>GPESQLDLRVQELIKLICNVQAMEEMMMEMKYNTKKAPLGKLTVAQIKAGYQSLKKIEDCIRAGQHGRALMEACNEFYTRIPHDFGLRTPPLIRTQKELSEKIQLLEALGDIEIAIKLVKSERQGLEHPLDQHYRNLHCALRPLDHESYEFKVISQYLQSTHAPTHSDYTMTLLDLFEVEKDGEKEAFREDLHNRMLLWHGSRMSNWVGILSHGLRIAPPEAPITGYMFGKGIYFADMSSKSANYCFASRLKNTGLLLLSEVALGQCNELLEANPKAEGLLQGKHSTKGLGKMAPSSAHFVTLNGSTVPLGPASDTGI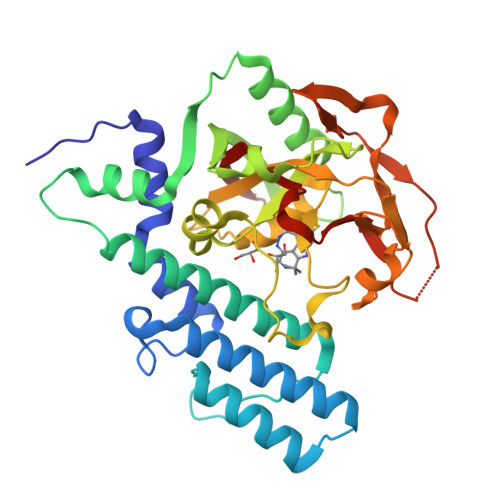LNPDGYTLNYNEYIVYNPNQVRMRYLLKVQFNFLQ[4x]>GHMSETNTIFKLEGVSVLSPLRKKLDLVFYLSNVDGSPVITLLKGNDRELSIYQLNKNIKMASFLPVPEKPNLIYLFMTYTSCEDNKFSEPVVMTLNKENTLNQFKKLGLLDSNVTDFEKCVEYIRKQAILTGFKISNPFVNSTLVDTDAEKINSFHLQCHRGTKEGTLYFL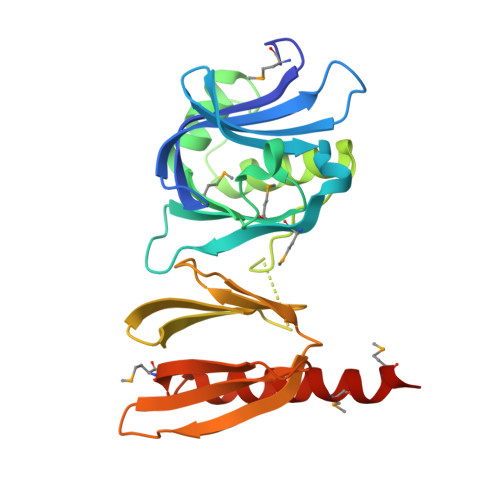PDHIIFGFKKPILLFDASDIESITYSSITRLTFNASLVTKDGEKYEFSMIDQTEYAKIDDYVKRKQMKDKSMSEELKAK[2x]The membrane-anchored SNARE (soluble N-ethylmaleimide-sensitive factor acceptor protein receptor) proteins provide the energy to drive membrane fusion in various cellular contexts, such as intracellular trafficking and exocytosis. Supercomplexes of NSF, α-SNAP, and either a syntaxin tetramer or one of two binary complexes of syntaxin—SNAP-25 reveal atomic details of SNARE processing and show how sequential ATP hydrolysis drives disassembly. NSF comprises three structured domains connected by flexible linkers—the adapter N-domain followed by the D1 and D2 AAA+ domains. Six NSF protomers come together to form the active form of the enzyme, a homo-hexamer.

The remaining 59% of particles were SNARE-substrate free and grouped into three classes with split D1 and D2 rings; presumably, this is a post-disassembly, substrate-released state, and it is not observed under non-hydrolyzing conditions. The particles show a population shift towards a flatter D1 ring that is closer to D2 relative to the non-hydrolyzing class. This is particularly clear in the case of the SNARE-substrate free classes, which also show an expanded pore. Finally, substrate-free classes are always ADP bound, even in protomer E; they are flat, have some N-domains packed between the D1 and D2 rings, and are characterized by a split in both the D1 and D2 rings between protomers A and F (right column); this is consistent with a SNARE substrate side-loading mechanism proposed for the NSF ortholog in yeast, Sec1845. In the absence of a completely protomer F-rebound state in the hydrolyzing condition, however, we cannot distinguish between SNARE substrate rebinding before or after protomer E hydrolysis; the former case (ATP in fully rebound F and E) represents a classical “hand-over-hand” mechanism, while the latter case (ATP in fully rebound F, ATP ADP•Pi in E), a ratchet mechanism in which F re-engages substrate during or immediately following a translocation event driven by protomer E hydrolysis, locking in substrate translocation. The flattened D1 rings of the SNARE-substrate-free classes with ADP•Pi in protomers E are suggestive of the latter; flattening upon hydrolysis at protomer E could exert a pulling force on the substrate, and translocation would then take place with substrate engagement by a new protomer F and release of the old protomer A. Multiple rounds of translocation are expected to ultimately lead to melting of the engaged SNARE domain and subsequent disruption of the SNARE complex.

>[6x]GANMAGRSMQAARCPTDELSLSNCAVVSEKDYQSGQHVIVRTSPNHKYIFTLRTHPSVVPGSVAFSLPQRKWAGLSIGQEIEVALYSFDKAKQCIGTMTIEIDFLQKKNIDSNPYDTDKMAAEFIQQFNNQAFSVGQQLVFSFNDKLFGLLVKDIEAMDPSILKGEPASGKRQKIEVGLVVGNSQVAFEKAENSSLNLIGKAKTKENRQSIINPDWNFEKMGIGGLDKEFSDIFRRAFASRVFPPEIVEQMGCKHVKGILLYGPPGCGKTLLARQIGKMLNAREPKVVNGPEILNKYVGESEANIRKLFADAEEEQRRLGANSGLHIIIFDEIDAICKQRGSMAGSTGVHDTVVNQLLSKIDGVEQLNNILVIGMTNRPDLIDEALLRPGRLEVKMEIGLPDEKGRLQILHIHTARMRGHQLLSADVDIKELAVETKNFSGAELEGLVRAAQSTAMNRHIKASTKVEVDMEKAESLQVTRGDFLASLENDIKPAFGTNQEDYASYIMNGIIKWGDPVTRVLDDGELLVQQTKNSDRTPLVSVLLEGPPHSGKTALAAKIAEESNFPFIKICSPDKMIGFSETAKCQAMKKIFDDAYKSQLSCVVVDDIERLLDYVPIGPRFSNLVLQALLVLLKKAPPQGRKLLIIGTTSRKDVLQEMEMLNAFSTTIHVPNIATGEQLLEALELLGNFKDKERTTIAQQVKGKKVWIGIKKLLMLIEMSLQMDPEYRVRKFLALLREEGASPLDFD> MEGGKLQSTFVFEEIGRRLKDIGPEVVKKVNAVFEWHITKGGNIGAKWTIDLKSGSGKVYQGPAKGAADTTIILSDEDFMEVVLGKLDPQK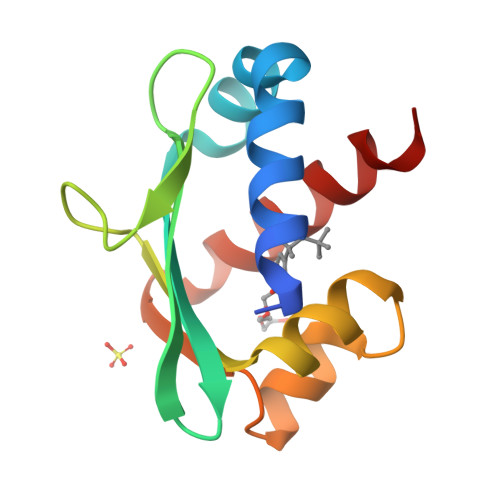AFFSGRLKCRGNIMLSQKLQMILKDYAKL>WQENKSWNAHFTEHKSQGVVVLWNENKQQGFTNNLKRANQAFLPASTFKIPNSLIALDLGVVKDEHQVFKWDGQTRDIATWNRDHNLITAMKYSVVPVYQEFARQIGEARMSKMLHAFDYGNEDISGNVDSFWLDGGI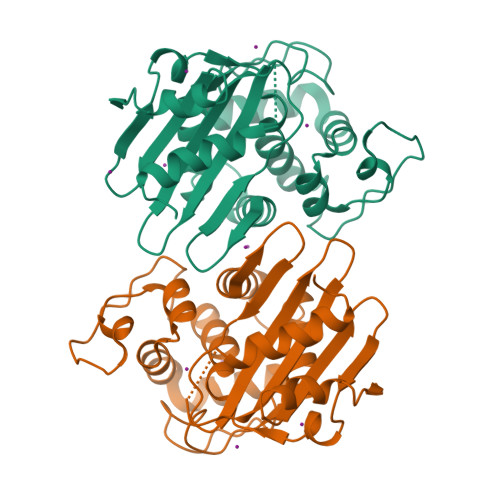RISATEQISFLRKLYHNKLHVSERSQRIVKQAMLTEANGDYIIRAKTGYDTKIGWWVGWVELDDNVWFFAMNMDMPTSDGLGLRQAITKEVLKQEKIIP[4x]> ASWSHPQFEKGASGAAESKPTPQSTFTGPIVVDPITRIEGHLRIMVEVENGKVKDAWSSSQLFRGLEIILKGRDPRDAQHFTQRACGVCTYVHALASSRCVDDAVKVSIPANARMMRNLVMASQYLHDHLVHFYHLHALDWVDVTAALKADPNKAAKLAASIAPARPGNSAKALKAVQDKLKAFVESGQLGIFTNAYFLGGHKAYYLPPEVDLIATAHYLEALHMQVKAASAMAILGGKNPHTQFTVVGGCSNY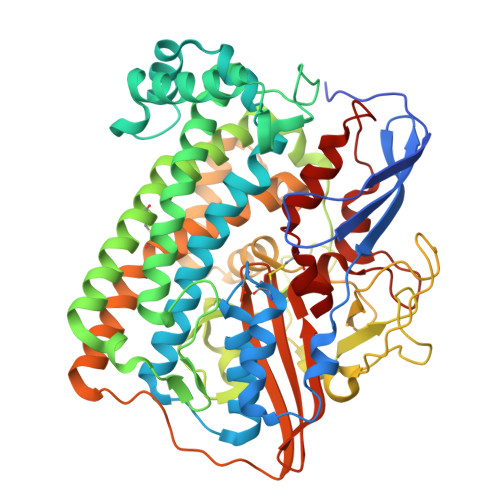QGLTKDPLANYLALSKEVCQFVNECYIPDLLAVAGFYKDWGGIGGTSNYLAFGEFATDDSSPEKHLATSQFPSGVITGRDLGKVDNVDLGAIYEDVKYSWYAPGGDGKHPYDGVTDPKYTKLDDKDHYSWMKAPRYKGKAMEVGPLARTFIAYAKGQPDFKKVVDMVLGKLSVPATALHSTLGRTAARGIETAIVCANMEKWIKEMADSGAKDNTLCAKWEMPEESKGVGLADAPRGALSHWIRIKGKKIDNFQLVVPSTWNLGPRGAQGDKSPVEEALIGTPIADPKRPVEILRTVHAFDPCIACGVH>GSMKKEFTELYDFIFDPIFLVRYGYYDRSIKNKKMNTAKVELDNEYGKSDSFYFKVFNMESFADYLRSHDLKTHFNGKKPLSTDPVYFNIPKNIEARRQYKMPNLYSYMALNYYICDNKKEFIEVFIDNKFSTSKFFNQLNFDYPKTQEITQTLLYGGIKKLHLDLSNFYHTLYTHSIPWMIDGKSASKQNRKKGFSNTLDTLITACQYDETHGIPTGNLLSRIITELYMCHFDKQMEYKKFVYSRYVDDFIFPFTFENEKQEFLNEFNLICRENNLIINDNKTKVDNFPF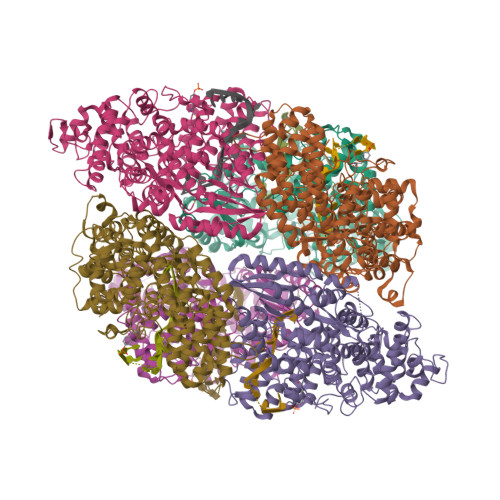VDKSSKSDIFSFFENITSTNSNDKWIKEISNFIDYCVNEEHLGNKGAIKCIFPVITNTLKQKKVDTKNIDNIFSKRNMVTNFNVFEKILDLSLKDSRLTNKFLTFFENINEFGFSSLSASNIVKKYFSNNSKGLKEKIDHYRKNNFNQELYQILLYMVVFEIDDLLNQEELLNLIDLNIDDYSLILGTILYLKNSSYKLEKLLKKIDQLFINTHANYDVKTSRMAEKLWLFRYFFYFLNCKNIFSQKEINSYCQSQNYNSGQNGYQTELNWNYIKGQGKDLRANNFFNELIVKEVWLISCGENEDFKYLN[6x]Within this system, SP represents the preferred endogenous agonist of NK1R4. Here, we report three crystal structures of the human NK1R bound to CP-99,994 and the clinically approved antagonists aprepitant and netupitant at 3.27, 2.40 and 2.20 Å resolution, respectively. Overall, NK1R exhibits the canonical GPCR architecture comprising seven transmembrane helices (I–VII) with helix 8 lying parallel to the membrane plane. Taken together, the NK1R structures in complex with different antagonists capture the inactive receptor conformation.

Since the prototypical antagonist CP-99,994 already displays many chemical features that are relatively preserved in further developed compounds we initially solved the structure of NK1R in complex with this ligand. CP-99,994 specifically interacts with only seven residues from helices III to VI and one residue from ECL2 in NK1R. The core (2,3-cis-substituted-piperidine) is laterally wedged between the side chains of F2686.55 and Q1654.60 and capped by I182ECL2. Q1654.60 is positioned to concomitantly hydrogen-bond the piperidine core and the amine linker of arm 1. Mutation of Q1654.60 to either alanine, glutamic acid or aspartic acid severely reduce the binding affinity of CP-99,994. Arm 1 of CP-99,994 extends deep into the receptor core, exploiting a large, almost exclusively lipophilic groove at the base of the orthosteric pocket formed by M2917.39, M2957.43, M812.53, W2616.48, I2045.46, F2646.51 and P1123.32. Within this region, the aromatic methoxyphenyl group of arm 1 is wedged between F2646.51 and P1123.32 and sits above a deep protrusion into the receptor core. Arm 2 of CP-99,994 targets a second lipophilic sub-pocket, making hydrophobic contacts to I1133.33 and V2005.42, and is capped on top by a face-on π-stack with H1975.39. Mutation of H1975.39 to alanine attenuates binding affinity 3.5-fold, yet preserving the aromatic character of this residue by virtue of mutation to phenylalanine results in only a <2-fold reduction in binding affinity to the small molecule, supporting this observed π-π interaction with the receptor. While NK1R in complex with CP-99,994 crystallised in space group C2221, it is noteworthy that crystallisation of NK1R with both aprepitant and netupitant consistently lead to better diffracting crystals in a different condition belonging to space group P212121.

> MDNVLPVDSDLSPNISTNTSEPNQFVQPAWQIVLWAAAYTVIVVTSVVGNVVVMWIILAHKRMRTVTNYFLVNAAFAEASMAAFNTVVNFTYAVHNEWYYGLFYCKFHNFFPIAAIFASIYSMTAVAFDRYMAIIHPLQPRLSLTATKVVICVIWVLALLLAFPQGYYSTTETMPSRVVCKIEWPEHPNKIYEKVYHICVTVLIYFLPLLVIGYLYTVVGITLRASGIDCSFWNESYLTGSRDERKKSLLSKFGMDEGVTFMFIGRFDRGQKGVDVLLKAIEILSSKKEFQEMRFIIIGKGDPELEGWARSLEEKHGNVKVITEMLSREFVRELYGSVDFVIIPSYFEPFGLVALEAMCLGAIPIASAVGGLRDIITNETGILVKAGDPGELANAILKALELSRSDLSKFRENCKKRAMSFSEQVSAARKVVKMMIVVVCTFAICWLPFHIFFLLPYINPDLYLKKFIQQVYLAIMWLAMSSTMYNPIIYCCLNDRFRLGFKHAFRCCPFISAGDYEGLE> GPHMTDKSDRTDWVALMRAIRDHRDEAAFAELFQHFAPKVKGFLMKSGSVASQAEECAQDVMATVWQKAHLFDPSRASVATWIFTIARNRRIDGLR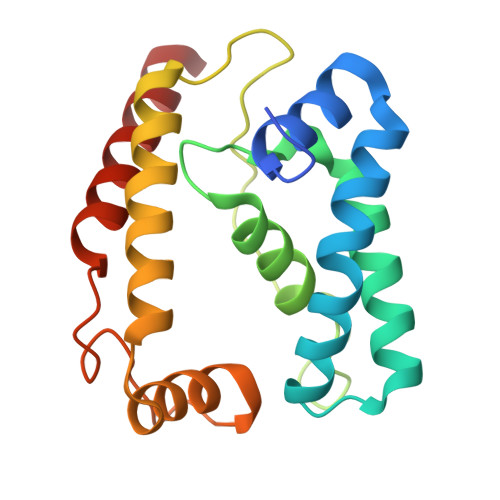KDRQPEPEDLFWGPDSEPDQADVYEMQQENARLGRAIARLPEAQRALIERAFFGDLTHRELAAETGLPLGTIKSRIRLALDRLRQHMS>[4x]MQKLLSLPSNLVQSFHELERVNRTDWFCTSDPVGKKLGSGGGTSWLLEECYNEYSDGATFGEWLEKEKRILLHAGGQSRRLPGYAPSGKILTPVPVFRWERGQHLGQNLLSLQLPLYEKIMSLAPDKLHTLIASGDVYIRSEKPLQSIPEADVVCYGLWVDPSLATHHGVFASDRKHPEQLDFMLQKPSLAELESLSKTHLFLMDIGIWLLSDRAVEILMKRSHKESSEELKYYDLYSDFGLALGTHPRIEDEEVNTLSVAILPLPGGEFYHYGTSKELISSTLSVQNKVYDQRRIMHRKVKPNPAMFVQNAVVRIPLCAENADLWIENSHIGPKWKIASRHIITGVPENDWSLAVPAGVCVDV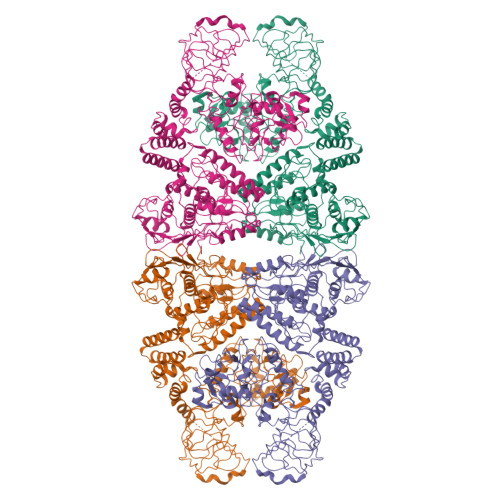VPMGDKGFVARPYGLDDVFKGDLRDSKTTLTGIPFGEWMSKRGLSYTDLKGRTDDLQAVSVFPMVNSVEELGLVLRWMLSEPELEEGKNIWLRSEHFSADEISAGANLKRLYAQREEFRKGNWKALAVNHEKSVFYQLDLADAAEDFVRLGLDMPELLPEDALQMSRIHNRMLRARILKLDGKDYRPEEQAAFDLLRDGLLDGISNRKSTPKLDVYSDQIVWGRSPVRIDMAGGWTDTPPYSLYSGGNVVNLAIELNGQPPLQVYVKPCKDFHIVLRSIDMGAMEIVSTFDELQDYKKIGSPFSIPKAALSLAGFAPAFSAVSYASLEEQLKDFGAGIEVTLLAAIPAGSGLGTSSILASTVLGAINDFCGLAWDKNEICQRTLVLEQLLTTGGGWQDQYGGVLQGVKLLQTEAGFAQSPLVRWLPDHLFTHPEYKDCHLLYYTGITRTAKGILAEIVSSMFLNSSLHLNLLSEMKAHALDMNEAIQRGSFVEFGRLVGKTWEQNKALDSGTNPPAVEAIIDLIKDYTLGYKLPGAGGGGYLYMVAKDPQAAVRIRKILTENAPNPRARFVEMTLSDKGFQVSRS>[2x]GYKERVERLCKSKELFEERLGLEIRRIHNEQLQFIFRHIDHKDPDKPYMFTLSINEQGDYEVTSCTPPLDCISEFQLKVRETNNFSAFIAN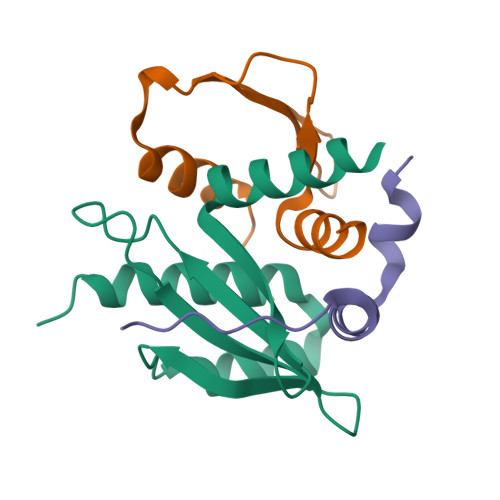IRKAFTALSFKQST;>[2x]GDEREDDGVPSAAYVTQLYYKISRIDWDYEVEPARIKGIHYGPDIAQPINMDSSHHSRCFISDYLWSLVPTAW;>[2x]GRNAFSELDSADPRVMLRRIIQNQPQVDPLALQTVQLEP>SVAADLPALPGGPAGGTGELAKYGLPGVAQLRSRESYVLSYDPRTRGALWVLEQLRPERLRGDGDRSACDFREDDSVHAYHRATNADYRGSGF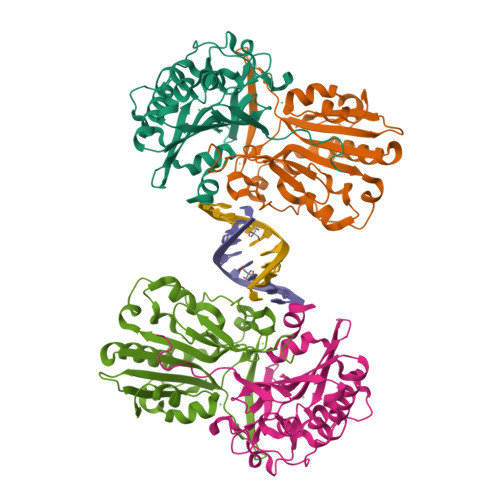DRGALAAAANHRWSQRAMDDTFYLSNVAPQVPHLNQNAWNNLERYSRSLTRTYQNVYVCTGPLFLPRTEADGKSYVKYQVIGKNHVAVPTHFFKVLILEAAGGQIELRSYVMPNAPVDETIPLERFLVPIESIERASGLLFVPNILARAGNLKAITAGSK[4x]> MASDYKDDDDKRRRGMEGAKLSAVRIAVREAPYRQFLGRREPSVVQFPPWSDGKSLIVDQNEFHFDHAFPATISQDEMYQALILPLVDKLLEGFQCTALAYGQTGTGKSYSMGMTPPGEILPEHLGILPRALGDIFERVTARQENNKDAIQVYASFIEIYNEKPFDLLGSTPHMPMVAARCQRCTCLPLHSQADLHHILELGTRNRRVRPTNMNSNSSRSHAIVTIHVKSKTHHSRMNIVDLAGSEGVRRTGHEGVARQEGVNINLGLLSINKVVMSMAAGHTVIPYRDSVLTTVLQASLTAQSYLTFLACISPHQCDLSETLSTLRFGTSAKKLRLEHHHH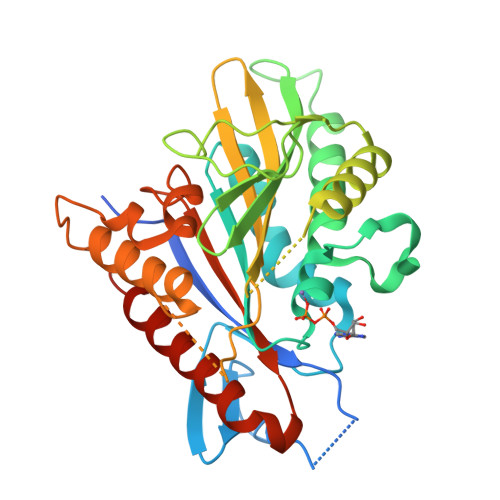HH HSF2BP is required for meiotic HR during spermatogenesis, but in somatic cells, it inhibits HR during DNA interstrand crosslink repair by triggering BRCA2 degradation. HSF2BP contains an N-terminal α-helical oligomerisation domain and a C-terminal domain predicted to adopt an Armadillo fold. We mapped the HSF2BP-BRCA2 interaction to the Armadillo domain of HSF2BP, and a 68 amino acid (aa) region of BRCA2 mostly encoded by exons 12 and 13, which is predicted to be disordered. In somatic animal cells, RAD51 loading onto ssDNA depends on BRCA2, which has multiple RAD51-binding sites and is required for focal accumulation of RAD51 at the sites of damage.

The crystal structure includes four ARM domains and two BRCA2 F15X peptides. The ARM domains A and D, as well as B and C, dimerize through a symmetric interface of about 950 Å2, formed by their N-terminal regions from E122 to I156. This interface is mediated by hydrophobic residues from helices α1, helices α2, and the N-terminus of helices α3. The BRCA2 peptide in orange (chain E) runs along the V-shaped groove formed by chains A and C. Similarly, the other BRCA2 peptide (in red; chain F) runs along the groove formed by chains B and D. At the center of the tetramer, a symmetric interface of about 250 Å2 is observed between the ARM domains A and B, which involves helices α2 and helices α5. In chains E and F, the N-terminal sequence, from N2291 to E2328, interacts with ARM domains C and D, respectively, whereas the C-terminal sequence, from D2312 to T2338, interacts with ARM domains A and B, respectively. BRCA2 motif 1, from N2291 to G2313, and BRCA2 motif 2, from T2314 to R2336, can be nicely superimposed, and interact with the same surface of their respective ARM domains. Sequence alignment between the two motifs identified five identical residues: D2294/2317, R2295/2318, S2303/2326 (also a proline in some organisms), L2304/2327, and P2311/2334, and two similar residues: A2306/P2329, S2309/C2332 (T2332 in our construct), which are all conserved through evolution. For example, D2294/2317 contacts R200 (helix α5) through a set of hydrogen bonds/salt bridges; R2295/2318 is hydrogen-bonded to S281 (helix α10); L2304/2327 contacts I242 (helix α7); S2309/C2332 and P2311/2334 interact W132 (helix α1); S2309/C2332 also contacts G188 and is hydrogen-bonded to N192 (helix α4). These conserved interactions between motif 1 and motif 2 of BRCA2 and two ARM monomers belonging to two different dimers trigger tetramerization of the ARM domain. The main contribution to the nanomolar affinity we measured comes from the large 2740 Å2 interface between one BRCA2 peptide and two HSF2BP ARM domains from two different ARM dimers.

>[4x]AEMGAAACTLLWGVSSSEEVVKAILGGDKALKFFSITGQTMESFVKSLDGDVQELDSDESQFVFALAGIVTNVAAIACGREFLVNSSRVLLDTILQLLGDLKPGQCTKLKVLMLMSLYNVSINLKGLKYISESPGFIPLLWWLLSDPDAEVCLHVLRLVQSVVLEPEVFSKSASEFRSSLPLQRILAMSKSRNPRLQTAAQELLEDLRTLEHNV;>[2x]NEFDRIIENQEKSLKASKSTPDGTIKDRRLFMHHVSLEPITTVPFRTTKERQENLYFQG> MGS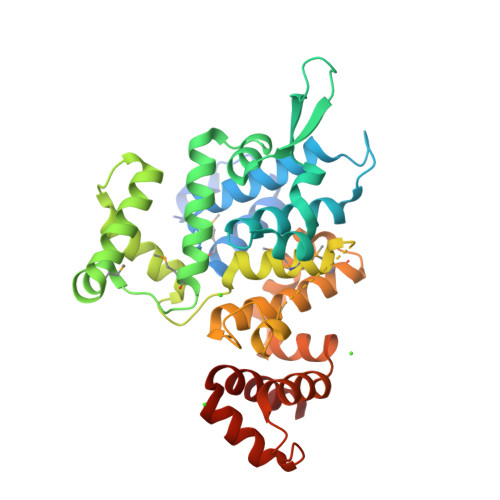SHHHHHHSQDPSDLSWSKRLSAYAALKDLTLSKQDKVFLEHLMTEYGFDSTTARQILKLKQGLERKFSSIFDDYTQEERDYLLFRIIGSVSYNGVKWDETAGYLSRYFYKEVVSNPVTGEKQKVPKSLLDIFQELGLSKAEAKQLQYNLSLQHEMAGGTLSTTGDMVKQDPDYYETAKNSYKLVYGTTEGFDKFWDERLKAYSNDGRGNADFTHQSITMATHLNPTSVQLSDIYGGRKHVKNLAGWEGDTTYNANERKPSIGEDDYKADLDSVNIIGRMKKGQSYQSAMSSYYSDVQKGHSVREKEFLKNKDWEKVKKTIYDSLVPNGINKNADSVVKDYIAKNYPDVSKFLSRLESVAGGQ>[2x]SDLIPAPPLSKVPLQQNFQDNQFHGKW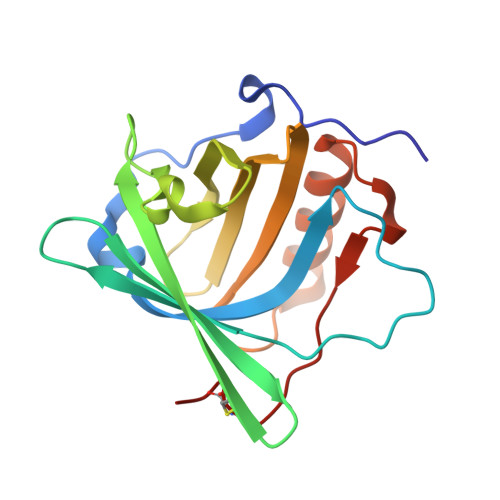YVVGFAENIQQREDKDPPKMIATIYELKEDKSYNVTNVASNWEKCTYRIKTFVPGSQPGEFTLGEIKSRPGMTSYLVRVVSTNYNQHAMVFFKTVVQNREKFWITLYGRTKELTSELKENFIRFSKSLGLPENHIVFPVPIDQCIDG> VDQATLDKLEAGFKKLQEASDCKSLLKKHLTKDVFDSIKNKKTGMGATLLDVIQSGVENLDSGVGIYAPDAESYRTFGPLFDPIIDDYHGGFKLTDKHPPKQWGDINTLVGLDPAGQFIISTRVRCGRSLQGYPFNPCLTAEQYKEMEEKVSSTLSS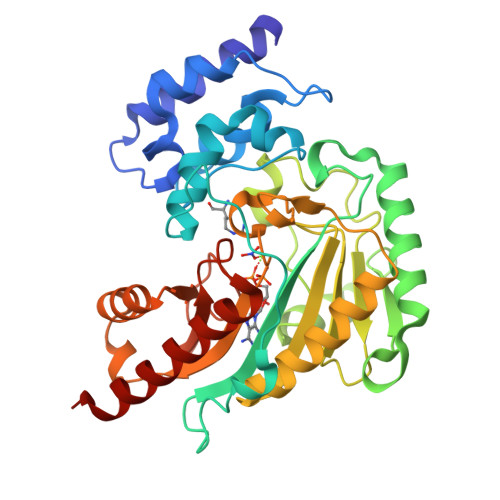MEDELKGTYYPLTGMSKATQQQLIDDHFLFKEGDRFLQTANACRYWPTGRGIFHNDAKTFLVWVNEQDHLRIISMQKGGDLKTVYKRLVTAVDNIESKLPFSHDDRFGFLTFCPTNLGTTMRASVHIQLPKLAKDRKVLEDIASKFNLQVRGTRGEHTESEGGVYDISNKRRLGLTEYQAVREMQDGILEMIKMEKAAA>[2x]HHNKVRTCWNEGRPALAGWLQLPGTLHAEALARLDYDAVVIDMQHSPIDFGQVAPMLIAIELGGAEPFVRTQVNDPSDIMKLLDAGAYGIIAPMVNTRAEAQTLASALHYSPRGLRSFGPRRPSLRYGSGYLAQASETVVGLAMIETREALANIDEILSVDGIDGVFIGPTDLALDLGHAPLVDTEEAEVVSAIAHVRERAHAAGKRVGIWCGSGGFARVKLAEGFDFVTAAPDLAMLSAAARQVIADARAL

Here structural analysis of hydroxyketoacid aldolase from Sphingomonas wittichii RW1 (SwHKA) revealed a dynamic movement of the metal cofactor between two coordination spheres without protein scaffold rearrangements. Holo‐SwHKA forms a trimer of homodimers, in which each monomer adopts an (α/β)8 triosephosphate isomerase (TIM) barrel fold. In total, holo‐SwHKA contains six equivalent active sites; each of which is formed from amino acids from two different domain‐swapped dimers. The transition from M2+ R to M2+ A,S is induced by bidentate substrate binding and occurs without a concomitant rearrangement of the protein scaffold.

In a previous study, several variants of SwHKA were created at position F210 in order to probe the influence of aromatic electron density for CH‐π interactions with hydroxypyruvate. In the absence of substrates, M2+ R constitutes the predominant state and the M2+ A,W complex was observed with lower occupancy in crystal structures of holo‐SwHKA.Here, we report the biochemical and structural characterization of OsUGT91C1, a glycosyltransferase from Oryza sativa, which is efficient at catalyzing β (1–2) glucosylation. OsUGT91C1 is able to catalyze the addition of both glucose 2-1-R1 and glucose 2-1-R2 with roughly equal efficiency. It also catalyzes a third reaction, β (1–6) glucose addition, to create previously uncharacterized compounds. The enzyme’s ability to bind steviol glycoside substrate in three modes underlies its flexibility to catalyze β (1–2) glucosylation in two distinct orientations as well as β (1–6) glucosylation.

The mutation of His27 to Ala completely inactivates OsUGT91C1 in β (1–2) glucosylation at either end of any previously assayed substrate. The inactivity of H27A and the single binding site for UDP leads to the conclusion that there is a single active site in the enzyme that catalyzes both glucose 2-1-R1 and 2-1-R2 addition. The H27A mutant is inactive, confirming that the cleavage arises from the same catalytic machinery of β (1–2) glucosylation. We managed to obtain the structure of the H27A inactivated mutant in a complex with Reb D and UDP. The Reb E complex indicated that glucose 2-1-R2 had been removed. The previously invisible glucose 2-1-R2 is well-ordered. Three complexes, native OsUGT91C1 with UDP and Reb E, native OsUGT91C1 with UDP and ST, and the H27A mutant with UDP and Reb D, bind steviol compounds with the R2 end at the active site. The trisaccharide attached to the R1 end of Reb D was built into a weak but unambiguous density. The same flip transition of glucose 1-R1 was also observed between the R1 tri-saccharides of Reb D and Reb E.

> MDSGYSSSYAAAAGMHVVICPWLAFGALLPCLDLAQRLASRGHRVSFVSTPRNISRLPPVRPALAPLVAFVALPLPRVEGLPDGAESTNDVPHDRPDMVELHRRAFDGLAAPFSEFLGTACADWVIVDVFHHWAAAAALEHKVPCAMMLLGSAHMIASIADRRLERAETESPAAAGQGRPAAAPTFEVARMKLIRTKGSSGMSLAERFSLTLSRSSLVVGRSCVEFEPETVPLLSTLRGKPITFLGLMPPLHEGRREDGEDATVRWLDAQPAKSVVYVALGSEVPLGVEKVHELALGLELAGTRFLWALRKPTGVSDADLLPAGFEERTRGRGVVATRWVPQMSILAHAAVGAFLTHCGWNSTIEGLMFGHPLIMLPIFGDQGPNARLIEAKNAGLQVARNDGDGSFDREGVAAAIRAVAVEEESSKVFQAKAKKLQEIVADMACHERYIDGFIQQLRSYKDLEHHHHHH> MHHHHHHAVRASEISRVYEAYPEKKATLYFLVLGFLALIVGSLFGPFQALNYGNVDAYPLLKRLLPFVQSYYQGLTLHGVLNAIVFTQLFAQAIMVYLPARELNMRPNMGLMWLSWWMAFIGLVVAALPLLANEATVLYTFYPPLKGHWAFYLGASVFVLSTWVSIYIVLDLWRRWKAANPGKVTPLVTYMAVVFWLMWFLASLGLVLEAVLFLLPWSFGLVEGVDPLVARTLFWWTGHPIVYFWLLPAYAIIYTILPKQAGGKLVSDPMARLAFLLFLLLSTPVGFHHQFADPGIDPTWKMIHSVLTLFVAVPSLMTAFTVAASLEFAGRLRGGRGLFGWIRALPWDNPAFVAPVLGLLGFIPGGAGGIVNASFTLDYVVHNTAWVPGHFHLQVASLVTLTAMGS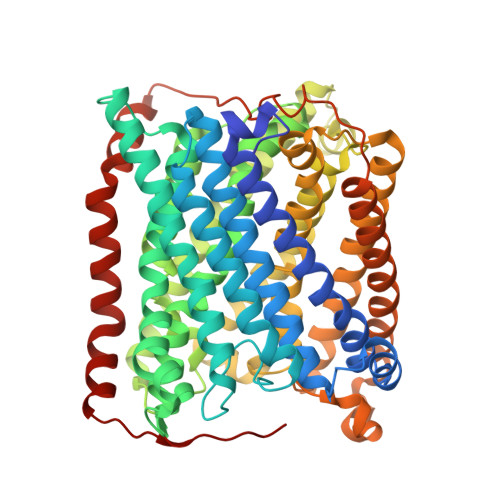LYWLLPNLTGKPISDAQRRLGLAVVWLWFLGMMIMAVGLHWAGLLNVPRRAYIAQVPDAYPHAAVPMVFNVLAGIVLLVALLLFIYGLFSVLLSRERKPELAEAPLPFAEVISGPEDRRLVLAMDRIGFWFAVAAILVVLAYGPTLVQLFGHLNPVPGWRLW> MRHRGGRG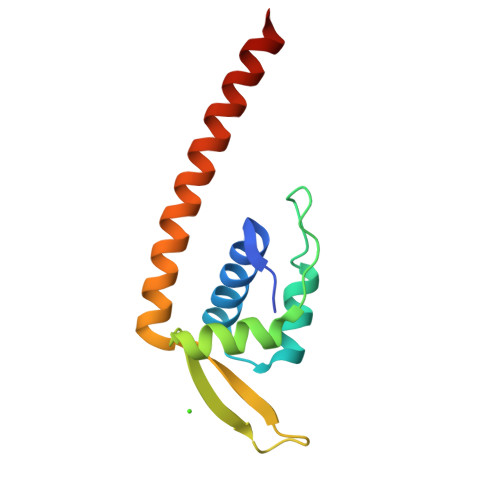FRGWWLASTILLLVAEKPSHGYELAERLAEFGIEIPGIGHMGNIYRVLADLEESGFLSTEWDTTVSPPRKIYRITPQGKLYLREILRSLEDMKRRIETLEERIKRVLQEE> HAEGTFTSDVSSYLEG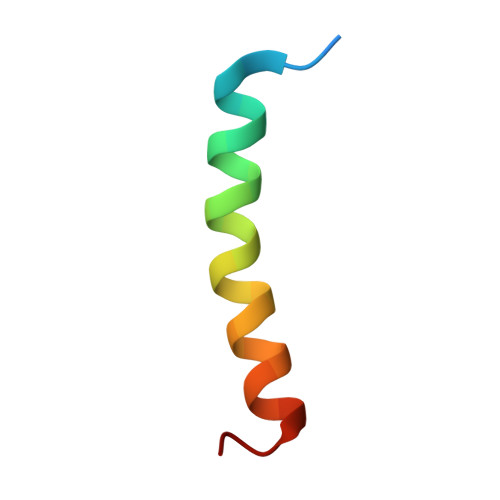QAAKEFIAWLVRGRG> GAPATVTEQGEDITSKKDRGVLKIVKRVGNGEETPMIGDKVYVHYKGKLSNGKKFDSSHDRNEPFVFSLGKGQVIKAWDIGVATMKKGEICHLLCKPEYAYGSAGSLPKIPSNATLFFEIELLDFKGE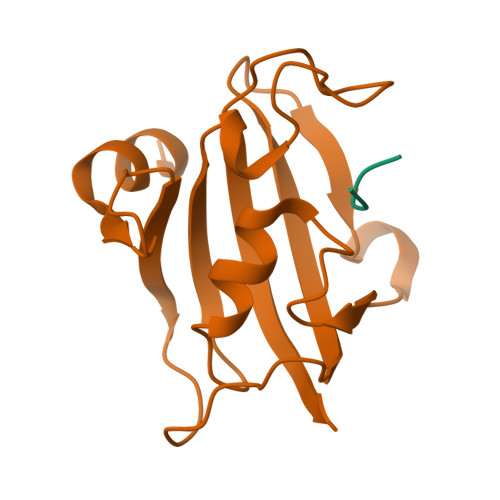;> SFPFT> MVDYIVEYDYDAVHDDELTIRVGEIIRNVKKLQEEGWLEGELN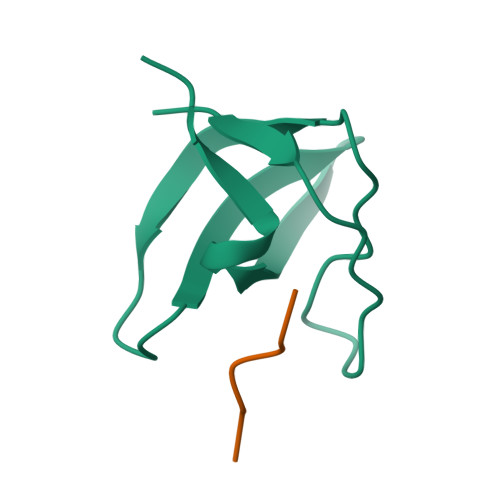GRRGMFPDNFVKEIKRETE;> KGPPLPRPRV> GSNEKAVILDEQAIRRALTRIAHEIIERNKG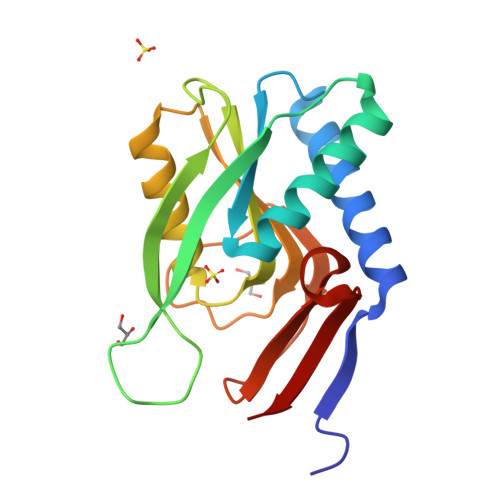VDNCVLVGIKTRGIYLAKRLAERIEQIEGKPVPVGEIDITLYRDDLSVTSNDEPLVKGTDIPVDITDKKVILVDDVLYTGRTVRAGMDALMDLGRPSQIQLAVLVDRGHRELPIRADYVGKNVPTSKSERIVVQLDEVDQNDRVSIYEN> GGFYEIEAIRRKRVRKGKVQYLIKWRGWPETANTWEPLENLQSIADVIDAFEGSLK;> QT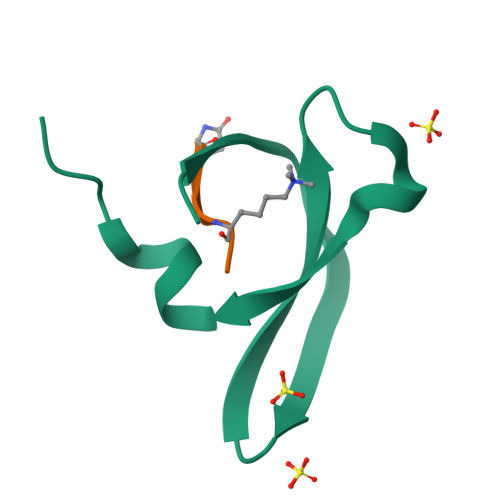ARKS>[2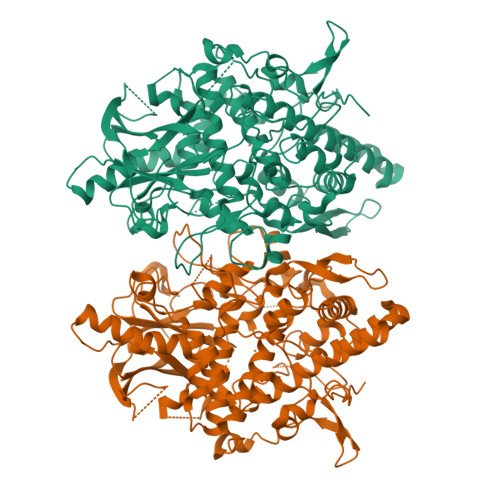x]GPGGSPYLITGIPKDPKHPLPIRKDIDDWYLEQTSAGSNRIQLTLFVEALTVIQNRPLNDQLSYFRLAGIHGAPWTEWDGVPGGQKDSKGNPTGFCVHNNYTFPTWHRVYVTLYEQVIYEAMLDFIKQNVPQNGKADWENEAKQWRLPYWDFARFARHGHDNTQGDELRLPILVTMPMVKVLVPGQPGKQLSKPNPLYRFQMQTLMGTLERPYAITSQKTEEHGWSFDLPFDKCQSTTKYGLLENYNADVWADGGQNWLRANLALNEHPWYQNLDGWDSVPTLQDMTFRLLTTGGLNWGEFSSTRYDDKKEETQPKNNEQAPKNWMNLEAIHNNVHNWVGGFMFSRPGRHDLKLWGAGHMSSVPVAAYDPIFWLHHCNIDRLTAIWQTVNSGSWFNDDKSKVSKDDDLRPFHRFCEKTRKVVFFRSDDVKDWRSLNYDYAITKDASRIRKEISDLYGQRTKEVYKDFGEEDYILSIRYSRYALGGKPFQINIFFGDVDGKDFYDARSQNFVGSVFNFSGSLEDSNCDKCAQQEQEGVLSVSQLPARLAVHYYKKQNKGEVPTPRYVVVNSQGKAEAEVKVEVALHKTEGTFYDAPARGGSDDYRRVADGKRAEVDDAYRA> GDLADRFAELERRYDARLGVYVPATGTTAAIEYRADERFAFCSTFKAPLVAAVLHQNPLTHLDKLITYTSDDIRSISPVAQQHVQTGMTIGQLCDAAIRYSDGTAANLLLADLGGPGGGTAAFTGYLRSLGDTVSRLDAEEPELNRDPPGDERDTTTPHAIALVLQQLVLGNALPPDKRALLTDWMARNTTGAKRIRAGFGADWKVIDKTGTGDYGRANDIAVVWSPTGVPYVVAVMSDRAGGGYDAEPREALLAEAATCVAGVLA

We investigated the roles of three conserved prolines at positions 107, 226, and 258 in the β‐lactamase BlaC from Mycobacterium tuberculosis and found that mutations can lead to dimerization of the enzyme and an overall less stable protein that is prone to aggregate over time. BlaC has 15 proline residues but only these three are 97%–99% conserved among class A β‐lactamases (Armon et al., 2001; Ashkenazy et al., 2010; Berezin et al., 2004). In this study, we investigated the effects of substitutions on the structure, activity, and stability of BlaC. It was found that substitutions in all three prolines lead to an overall less stable enzyme, more prone to oligomerization and aggregation. We propose that one of the roles of conserved prolines in BlaC is to prevent protein association and maintain the monomeric state.

Pro226 is found in a loop between β‐strand 3 and an α‐helix in an α/β‐domain, interacting with Trp229, another highly conserved residue. The crystal structure of BlaC P226G solved to 1.3 Å displays virtually no differences to the structure of wild‐type BlaC, with average Cα RMSD of 0.34 Å. Surprisingly, even the loop containing residue 226 displayed no changes. The absence of the pyrrolidine ring allowed for an additional ordered water to be present in a mutant structure. For BlaC Pro226 variants, the structures closely resemble that of wild‐type BlaC. Changes in NMR resonances of amides were localized around the mutation site and virtually no changes were found in the crystal structure. It is plausible that this highly conserved proline located in the loop limits protein dynamics. For Pro226 variants, T m values were about 2 degrees lower than for wild type, and for Pro258 variants, T m changes were small, indicating that both these residues are unlikely to be essential for the thermal stability.> LCT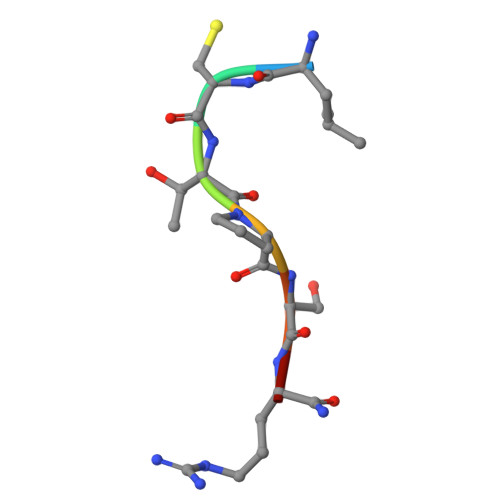PSRA> MQNSALKAWLDSSYLSGANQSWIEQLYEDFLTDPDSVDANWRSTFQQLPGTGVKPDQFHSQTREYFRRLAKDASRYSSTISDPDTNVKQVKVLQLINAYRFRGHQHANLDPLGLWQQDKVADLDPSFHDLTEADFQETFNVGSFASGKETMKLGELLEALKQTYCGPIGAEYMHITSTEEKRWIQQRIESGRATFNSEEKKRFLSELTAAEGLERYLGAKFPGAKRFSLEGGDALIPMLKEMIRHAGNSGTREVVLGMAHRGRLNVLVNVLGKKPQDLFDEFAGKHKEHLGTGDVKYHMGFSSDFQTDGGLVHLALAFNPSHLEIVSPVVIGSVRARLDRLDEPSSNKVLPITIHGDAAVTGQGVVQETLNMSKARGYEVGGTVRIVINNQVGFTTSNPLDARSTPYCTDIGKMVQAPIFHVNADDPEAVAFVTRLALDFRNTFKRDVFIDLVCYRRHGHNEADEPSATQPLMYQKIKKHPTPRKIYADKLEQEKVATLEDATEMVNLYRDALDAGDCVVAEWRPMNMHSFTWSPYLNHEWDEEYPNKVEMKRLQELAKRISTVPEAVEMQSRVAKIYGDRQAMAAGEKLFDWGGAENLAYATLVDEGIPVRLSGEDSGRGTFFHRHAVIHNQSNGSTYT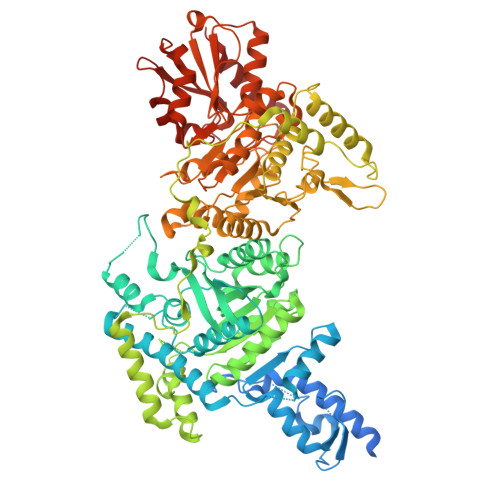PLQHIHNGQGAFRVWDSVLSEEAVLAFEYGYATAEPRTLTIWEAQFGDFANGAQVVIDQFISSGEQKWGRMCGLVMLLPHGYEGQGPEHSSARLERYLQLCAEQNMQVCVPSTPAQVYHMLRRQALRGMRRPLVVMSPKSLLRHPLAVSSLEELANGTFLPAIGEIDELDPKGVKRVVMCSGKVYYDLLEQRRKNNQHDVAIVRIEQLYPFPHKAMQEVLQQFAHVKDFVWCQEEPLNQGAWYCSQHHFREVIPFGASLRYAGRPASASPAVGHMSVHQKQQQDLVNDALNVE BIPHENYL-2,3-DIOL | 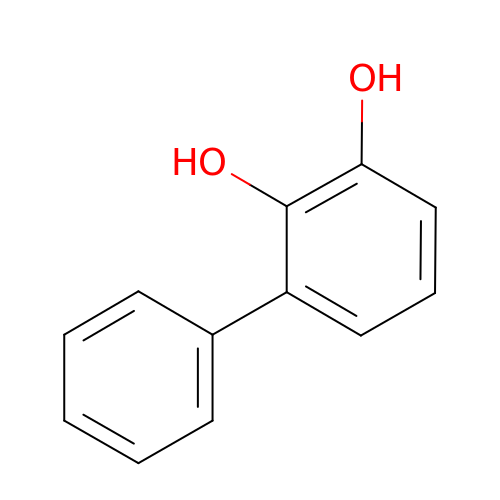C12 H10 O2 | YKOQAAJBYBTSBS-UHFFFAOYSA-N2-(2-((benzofuran-2-carboxamido)methyl)-5-methoxy-1H-indol-1-yl)acetic 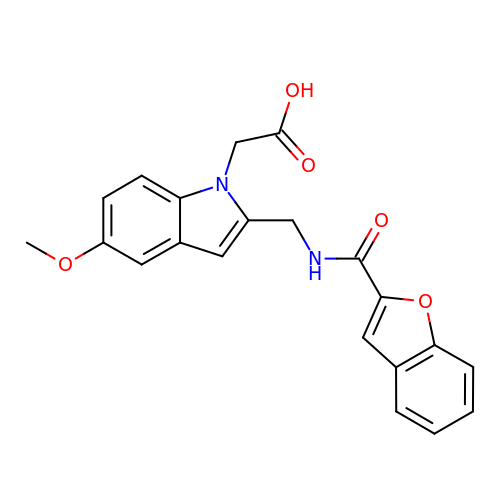acid | C21 H18 N2 O5 | CYMXZVQAGCGDHU-UHFFFAOYSA-N> VSTLIPPKVVSSKNIGSAPNAKRIANVVHFYKSLPQGPAPAIKANTRLARYKAKYFDGDNAS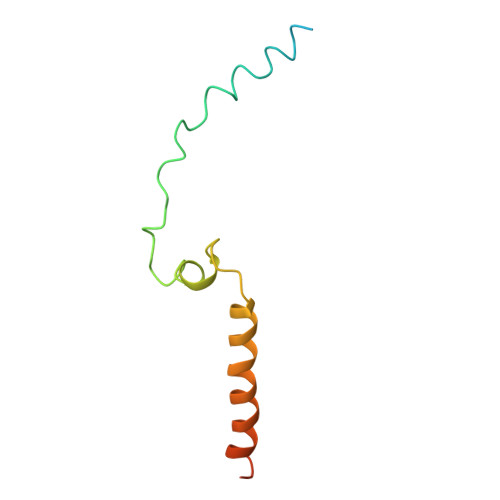GKPLWHFALGIIAFGYSMEYYFHLRHHKGAEEH>[2x]GSHMVIPAGKLERVDPTTVRQEGPWA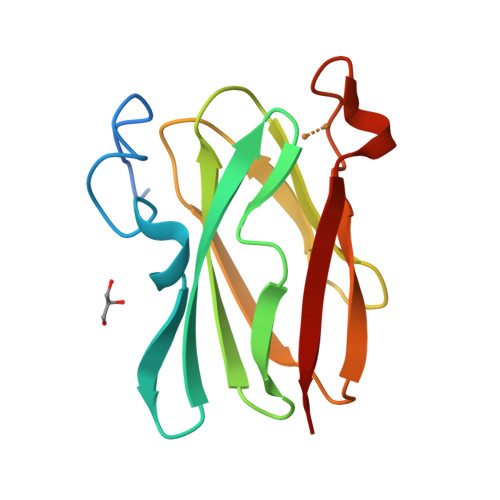DPAQAVVQTGPNQYTVYVLAHQWYYQPNPIEVPQGAEIVFKITSQDVLHGFHVEGTNINVEVLPGEVSTVRYTFKRPGEYRIICSEICGANHSNMFGTIVVKE Aminoacyl-tRNA synthetases (AARSs) attach amino acids to their corresponding tRNA adaptors with high specificity in an essential reaction of protein synthesis. An angiogenic role has recently been identified for the class II threonyl-tRNA synthetase (TARS for eukaryotes; ThrRS for prokaryotic orthologs) that is distinct from those of YARS and WARS. TARS is secreted from endothelial cells in response to TNF-α and VEGF, and potently stimulates angiogenesis in the human umbilical vein endothelial cell (HUVEC) tube formation and chicken chorioallantoic membrane assays. The isolation of resistant bacterial strains2627 and Chinese hamster ovary cell lines with selective gene amplification demonstrated that the principal target of borrelidin in bacteria and eukaryotes is threonyl-tRNA synthetase.

As a first step towards understanding the molecular basis of these effects, we co-crystallized BC194 with a fragment of human TARS comprising the catalytic and anticodon binding domains, and solved the structure to a resolution of 2.8 Å. The structures of BN and BC194 differ at position C17, with BN containing a pendant cyclopentanecarboxylic acid ring, and BC194 a cyclobutanecarboxylic acid ring. BC194 binding to the TARS active site is stabilized by numerous Van der Waals interactions and five distinct enzyme-compound hydrogen bonds. In addition, BC194 induces a conformation of TARS close to that of BN – TARS complex, with an r.m.s.d. of 0.62 Å between superimposed BC194 and BN – TARS complex structures (for all 402 Ca’s in TARS). Interactions between TARS and the C4 to C14 moiety of the macrolide structure are conserved in the BN and BC194-TARS complexes, including hydrophobic contacts to the macrolide ring made by L567, S386, H388, Y540, D564, Q562, H590, Y392, H391, and F539. In complexes with both compounds, residues T560, R442, M411, C413, Q460 and A592 comprise a binding pocket outside the macrolide ring, and interact with the C17 cyclobutanecarboxylic acid ring. The key structural difference that differentiates how BN and BC194 interact with TARS is seen in the contacts made to the respective pendant rings. In the BC194 complex, the absence of a methylene group in the smaller cyclobutane ring lengthens the contact between the C17 carboxylic-oxygen atom and the 5-amide nitrogen atom of Q460 by 0.9 Å. A strong hydrogen bond normally found in the BN complex is eliminated, and the hydrophobic interaction between the cyclopentane ring and A592 is also weakened. The loss of the interactions with these two residues suggests that BC194 may compete less effectively against threonine for binding than the parent compound BN.

>[4x]MGSSHHHHHHSSDHRKIGRDQELYFFHELSPGSCFFLPKGAYIYNALIEFIRSEYRKRGFQEVVTPNIFNSRLWMTSGHWQHYSENMFSFEVEKELFALKPMNCPGHCLMFDHRPRSWRELPLRLADFGVLHRNELSGALTGLTRVRRFQQDDAHIFCAMEQIEDEIKGCLDFLRTVYSVFGFSFKLNLSTRPEKFLGDIEVWDQAEKQLENSLNEFGEKWELNSGDGAFYGPKIDIQIKDAIGRYHQCATIQLDFQLPIRFNLTYVSHDGDDKKRPVIVHRAILGSVERMIAILTENYGGKWPFWLSPRQVMVVPVGPTCDEYAQKVRQQFHDAKFMADIDLDPGCTLNKKIRNAQLAQYNFILVVGEKEKISGTVNIRTRDNKVHGERTISETIERLQQLKEFRSKQAEEEF> AHHHHHHVDDDDKMIEMIATTMSVPRQVEVTEKFKSLVTAHNGKDEEMKDVAQDMKNYMDEKYGRVWQCVILTGSYWMHFSHE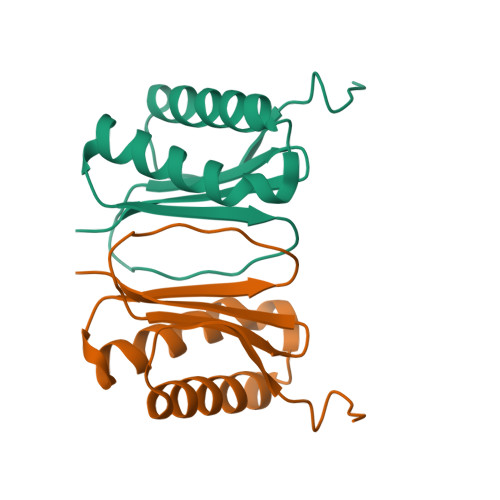PFLSIQFRYGRHICLAWRTPRG>[2x]MVEIPAIDLRLAGGGGGAEETARLRDACARLGCFRVSGHGVPPGLQAEMKAAVRALFDLPDDAKRRNADIIPGSGYVPPGTANPLYEAFGLCDAAAPADVDAFCARLDAPPHVRETVKAYAERMHSLIVDVAGKVAASLGLHGASFQDWPCQFRMNRYNYTQDSVGSPGVQVHTDSGFLTVLQEDECVGGLEVLDPAAGEFVPVDPLPGSFVVNVGDVGQAWSNGRLHNV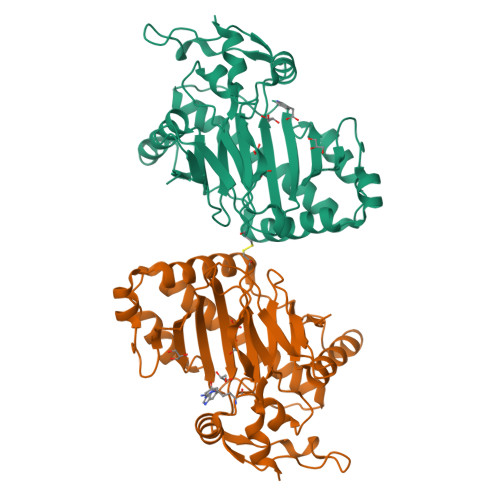KHRVQCVAAVPRVSIAMFLLAPKDDTVSAPGELVDGEHPRRYREFKYDDYRRLRLSTGERAGEALARLAA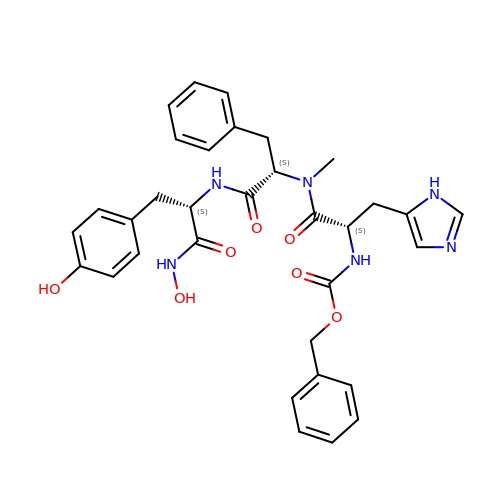N-[(benzyloxy)carbonyl]-L-histidyl-N-methyl-L-phenylalanyl-N-hydroxy-L-tyrosinamide | C33 H36 N6 O7 | SEPJJYNYJOZSET-AWCRTANDSA-N> GP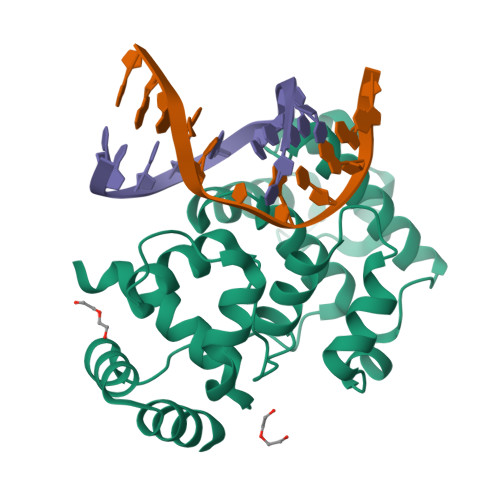GSMSKDSDYKRAEKHLSSIDNKWSSLVKKVGPCTLTPHPEHAPYEGIIRAITSQKLSDAATNSIINKFCTQCSDNDEFPTPKQIMETDVETLHECGFSKLKSQEIHIVAEAALNKQIPSKSEIEKMSEEELMESLSKIKGVKRWTIEMYSIFTLGRLDIMPADDSTLKNEAKEFFGLSSKPQTEEVEKLTKPCKPYRTIAAWYLWQIPKLHRKGQ> MPMISCDMRYGRTDEQKRALSAGLLRVISEATGEPRENIFFVIREGSGINFVQHGEHL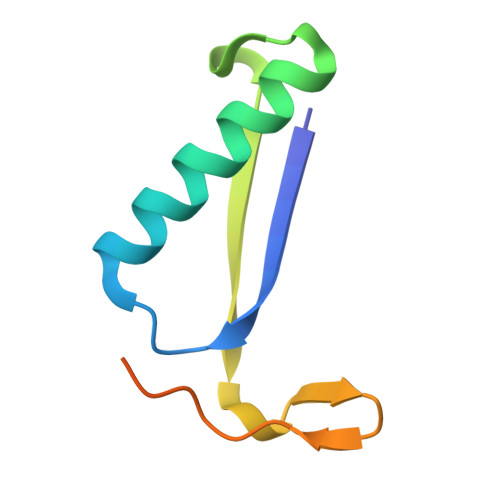PDYVPGNANDKALIAKLK>[2x]QVTVIPREQHAISRKDISENALKVMYRLNKAGYEAWLVGGGVRDLLLGKKPKDFDVTTNATPEQVRKLFRNCRLVGRRFRLAHVMFGPEIIEVATFRG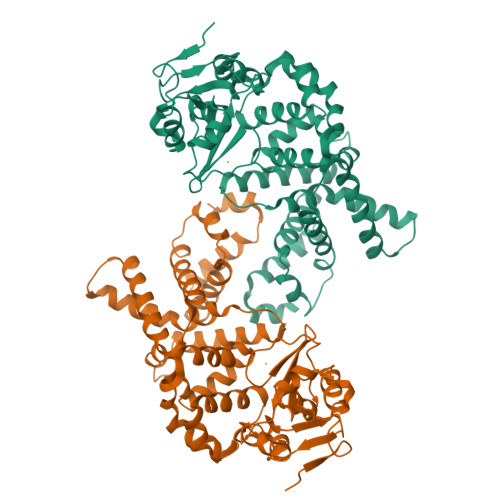HHEGNVSDRTTSQRGQNGMLLRDNIFGSIEEDAQRRDFTINSLYYSVADFTVRDYVGGMKDLKDGVIRLIGNPETRYREDPVRMLRAVRFAAKLGMRISPETAEPIPRLATLLNDIPPARLFEESLKLLQAGYGYETYKLLCEYHLFQPLFPTITRYFTENGDSPMERIIEQVLKNTDTRIHNDMRVNPAFLFAAMFWYPLLETAQKIAQESGLTYHDAFALAMNDVLDEACRSLAIPKRLTTLTRDIWQLQLRMSRRQGKRAWKLLEHPKFRAAYDLLALRAEVERNAELQRLVKWWGEFQVSAPPDQKGMLNELD>VRLPGLAAMRQGTRLFTPEQGEDLREALRRRRGSFQTT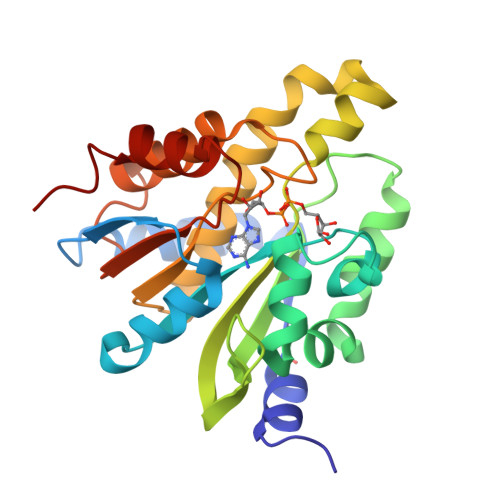CEVTSETTFAAARRLREKASALAALNFASAKNPGGGFLGGAQAQEEDLCRGSGLYFSLTSPQAEPYYAVNRQSHSALYTDHLIYSPQVPIFRDDAGQLLPAPVPVNIITAPAPNAGAVAQSRPEQLPQVLPTLRERARRVLGVAAWMEQTHLVLGAWGCGVFRNDPAGVARTFRELLEGEAQGAFEHVTFAVLDNHPQHPTLGAFRRELESLCLP[6x]> NADIYIPTLEEIKRTLQLAKDYSENV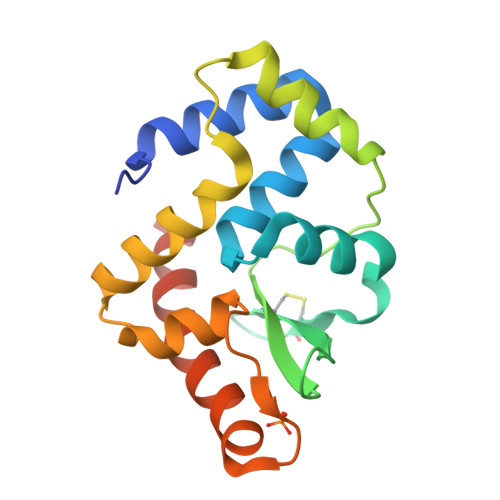YFIYRIALESGVRLSEVLKVLKEPERDICGNDVCYYPLSWTRGYKGVFYVFHITPLKRVEVTKWAIADFERRHKDAIAIKYFRKFVASKMAELSVPLDIIDFIQGRKPARVLTQHYVSLFGIAKEQYKKYAEWLKGVHHHHHH>MVKINFPILDEPLVLSNATILTIEDVSVYSSLVKHFYQYDVDEHLKLFDDKQKSLKATELMLVTDILGYDVNSAPILKLIHGDLENQFNEKPEVKSMVEKLAATITELIAFECLENELDLEYDEITILELIKALGVKIETQSDTIFEKCFEIIQVYHYLT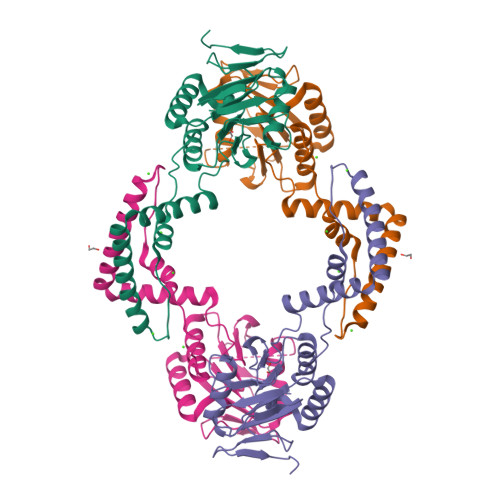KKNLLVFVNSGAYLTKDEVIKLCEYINLMQKSVLFLEPRRLYDLPQYVIDKDYFLIGENMVLEHHHHHH[2x]S-layer proteins (SLPs) are self-assembling, crystalline proteins coating the cell surfaces of many prokaryotes. We determined the atomic resolution structures of all functional domains (I-III from N- to C-termini) present in the three S-layer proteins SlpA_ac, SlpX_ac, and SlpA_amy. The Lactobacillus S-layers are anchored to the cell wall through interaction with teichoic acids (TA), either lipoteichoic acid (LTA) or wall teichoic acid (WTA).

The arrangement and architecture of SlpA_ac and SlpA_amy are highly similar. The N-terminal part, exhibiting the first two domains (SlpA_I and SlpA_II), is known to be responsible for the self-assembly of the S-layer protein into a regular lattice. The crystal structures of SlpA from L. acidophilus and L. amylovorus and observed crystal contacts reveal the self-assembly formation. A second interaction was observed within this crystal structure, a symmetrical homodimer interaction spanning from Asn92 to Asn176. The self-assembly region (SA) is formed by domains SlpA_I and SlpA_II, building a 2D crystalline network that forms the exposed surface of the SlpA layer.

>DVNTNIVLGGTTAPAVKGDVNVTSNVQAITSPQTTTIDNQTGAVTYSNWDGKVNGTVTATYNGQSYTATLNETAGKENSRVTPWYTQDGGKTWNVLKKDGGVYRLEPAGKYQLSVNNVSFNFGTANANKKNITLTSSNGVQFRENGQWKDSIKVSTDQNGAVSQPLTLLIPITPVDVTNAKS[2x]> MNIFRLTGDLSHLAAIIILLLKIWKSRSCAGISGKSQLLFALVFTTRYLDLFTSFISLYNTSMKLIYIACSYATVYLIYMKFKATYDGNHDTFRVEFLIVPVGGLSFLVNHDFSPLEILWTFSIYLESVAILPQLFMISKTGEAETITTHYLFFLGLYRALYLVNWIWRYYFEGFFDLIAVVAGVVQTVLYCDFFYLYVTKV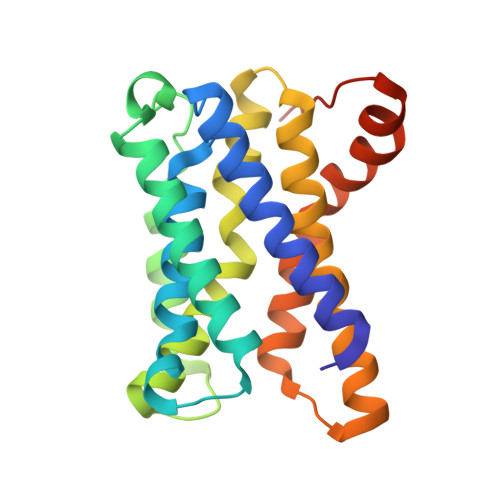LKGKKLSLPAGENLYFQ;> AERDEL> GPHMSTEKAPAALGPYSQAIKANNLVFLSGVLGLIPETGKFVSESVEDQTEQVLKNMGEILKASGADYSSVVKTTIMLADLADFKTVNEIYAKYFPAPSPA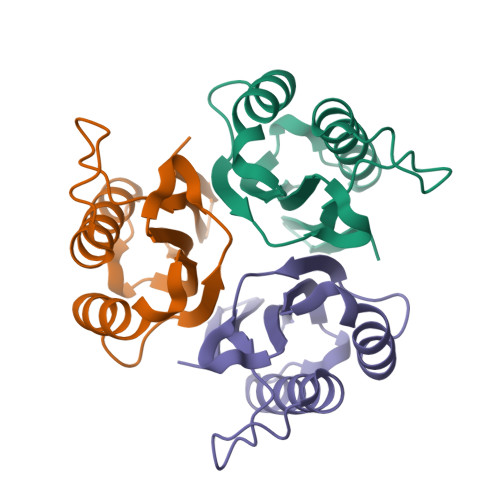RSTYQVAALPLNAKIEIECIATL>[2x]MHHHHHHAMNHETFLKRAVTLACEGVNAGIGGPFGAVIVKDGAIIAEGQNNVTTS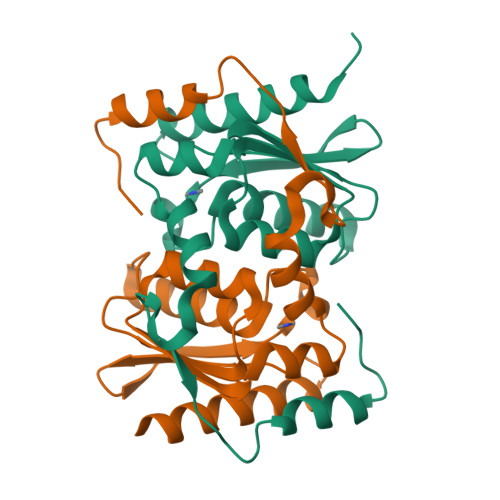NDPTAHAEVTAIRKACKVLGAYQLDDCILYTSCEPCPMCLGAIYWARPKAVFYAAEHTDAAEAGFDDSFIYKEIDKPAEERTIPFYQVTLTEHLSPFQAWRNFANKKEY>[2x]MGHHHHHHMLENIRDAVRKFLTGSTPYEKAVDEFIKDLQKSLISSDVNVKLVFSLT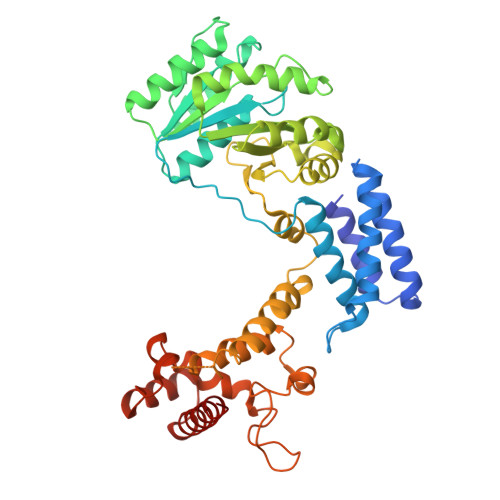AKIKERLNKEKPPSVLERKEWFISIVYDELSKLFGGDKEPNVNPTKLPFIIMLVGVQGSGKTTTAGKLAYFYKKRGYKVGLVAADVYRPAAYDQLLQLGNQIGVQVYGEPNNQNPIEIAKKGVDIFVKNKMDIIIVDTAGRHGYGEETKLLEEMKEMYDVLKPDDVILVIDASIGQKAYDLASRFHQASPIGSVIITKMDGTAKGGGALSAVVATGATIKFIGTGEKIDELETFNAKRFVSRILGMGDIESILEKVKGLEEYDKIQKKMEDVMEGKGKLTLRDVYAQIIALRKMGPLSKVLQHIPGLGIMLPTPSEDQLKIGEEKIRRWLAALNSMTYKELENPNIIDKSRMRRIAEGSGLEVEEVRELLEWYNNMNRLLKMVK> GAYKQVKLGEDAPNSSVVHVSNPESGNNYASEKTADGAECHLLDFASAERPLVVNFGSATCPPFTRQLPAFRQLVEEFSSVADFLLVYIDEAHPSD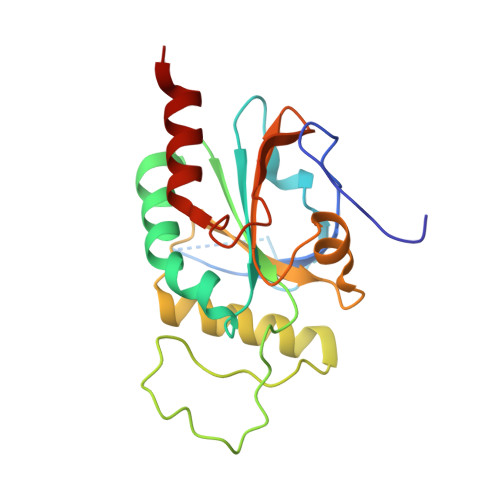GWAVPGDSSLSFEVAAHRNQEDRCAAAHQLLERFSLPPQCQVVADRMDNNANVAYGVAFERVCIVQRRKIAYLGGKGPFSYNLQEVRSWLEKNFSKR In 2020, Tan et al. discovered that BktB from Cupriavidus necator is a polyketoacyl-CoA thiolase and demonstrated its activity to produce polyketides, including TAL, through repetitive non-decarboxylative Claisen condensations with acetyl-CoA as both precursor and extension unit in vitro and in vivo in E. coli. One candidate, BktBbr from Burkholderia sp. RF2-non_BP3, exhibits approximately 30-fold higher activity in vitro and supports 30-fold higher TAL titers in Escherichia coli compared to the original enzyme. Additionally, we resolve the high-resolution X-ray structure of BktBbr with three different substrates: acetyl-CoA, acetoacetyl-CoA, and butyryl-CoA.

Comparing the apo structure with the structures covalently bound by CoA esters, no obvious structural changes were observed. Both acetyl-CoA and butyryl-CoA, acting as starter substrates for TAL and ketoacyl-CoA biosynthesis, respectively, displayed identical protein-ligand interactions: H-bonding between the keto group of substrates with C95 and G387 within the active pocket as well as interactions between the CoA with R226 and S254. Among the mutants, S254A, G255A, and G251A substantially boosted TAL production. A shared trait of these mutants was reduced CoA binding affinity in the substrate tunnel. S254A, located adjacent to the CoA tunnel as observed in the substrate-bound BktBbr structure, led to over a two-fold increase in TAL production, while S254C decreased it, implying that not just the water network but also CoA chain movement are vital for enzyme activity.

>[2x]GHMSNAAKEVVVVSGVRTAIGDFGGSLKDFSPTDLGAKVVSEVLSRANVSGDAVGHVVFGHVVNTEPKDMYLARVAAINGGVAQHTPALTVNRLCGSGLQAIVSAAQTIMLGDADVAIGGGSENMSRAPYTVPSARFGQRMGDAKLVDMMLGALHDPFQTIHMGVTAENVARKYGITRDAQDALALESHRRAARAIAEGRFKDQILPISIRTKKGEVAFDTDEHVRHDAGPDDFTKLKPVFVKEDGTVTAGNASGINDAAAAVLMMSADAARAQGVKPLARLVAYAHAGVDPAYMGIGPVPATQKALERAGLKITDLDVIEANEAFAAQACAVTQELGLDPAKVNPNGSGISLGHPIGATGALITVKALYELKRIGGRYALVTMCIGGGQGIAAIFENI>[3x]MFTGIITDIGKVDRVKPLNEGVLLR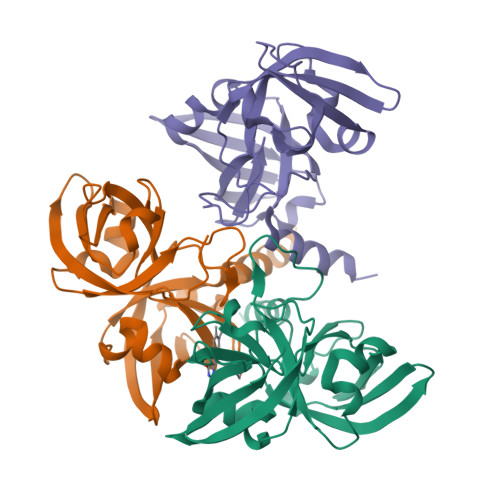IETAYDPETIELGASIACSGVCLTVVALPEKGSNARWFEVEAWEEALRLTTISSWQSGRKINLERSLKLGDEMGGHLVFGHVDGQAEIVERKDEGDAVRFTLRAPEELAPFIAQKGSVALDGTSLTVNGVNANEFDVLLIRHSLEVTTWGERKAGDKVNIEIDQLARYAARLAQYQKLEHHHHHH> GSHMERYDIAIIGSGPAGLASAINAKTRNKSVIVFGSSDLSKKLTLAPVINNYLGFYGIRGAELQEKFKEHIDNMGIQIENVKVNNIYAMGEYFSIMTSKDTYEASKVILAMGMEHTKPLKGEDKFLGRGVGYCATCDAPLYKGKIVTIVGYNKEAESEANYLAELASKVYYVPRYKDEYQLVSAVEIVKDVPVE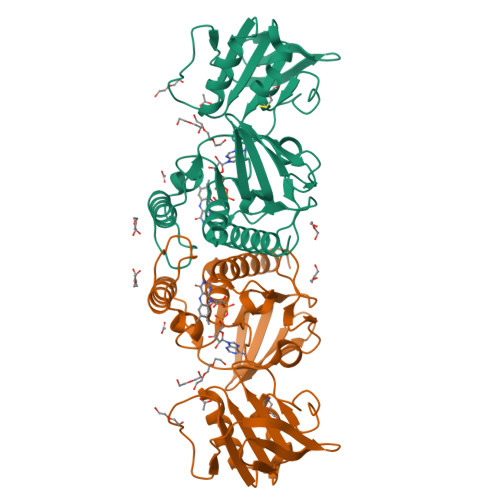IVGDKKVEKLKLKSRELETDGVFVLKDSAPPEQLVPGLYVEDGHIKVNRKMETNIDGCYAAGDCTGKPYQYMKAVGEGQVAALNAVEKLYTKA> AAAAAAAAAAAAAAAAAAAAAAAAAAAAAAAASLCLFPEDFLLKEFVEFF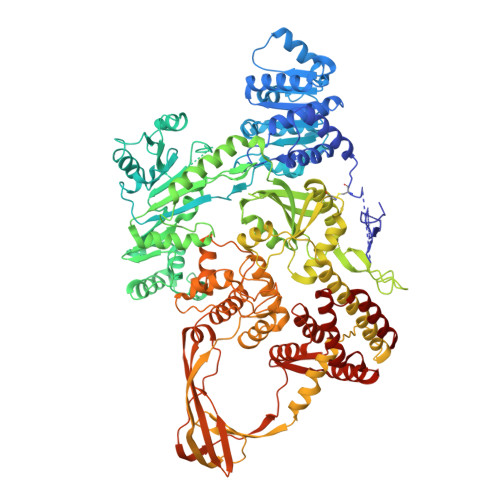RKCVGEPRAIQKMWAKRILRKESFAATAPTGVGKTSFGLAMSLFLALKGKRCYVIFPTSLLVIQAAETIRKYAEKAGVGTENLIGYYHGRIPKREKENFMQNLRNFKIVITTTQFLSKHYRELGHFDFIFVDDVDAILKASKNVDKLLHLLGFHYDLKTKSWVGEARGCLMVSTATAKKGKKAELFRQLLNFDIGSSRITVRNVEDVAVNDESISTLSSILEKLGTGGIIYARTGEEAEEIYESLKNKFRIGIVTATKKGDYEKFVEGEIDHLIGTAHYYGTLVRGLDLPERIRFAVFVGCPSFRVTIEDIDSLSPQMVKLLAYLYRNVDEIERLLPAVERHIDEVREILKKVMGKERPQAKDVVVREGEVIFPDLRTYIQGSGRTSRLFAGGLTKGASFLLEDDSELLSAFIERAKLYDIEFKSIDEVDFEKLSRELDESRDRYRRRQEFDLIKPALFIVESPTKARQISRFFGKPSVKVLDGAVVYEIPMQKYVLMVTASIGHVVDLITNRGFHGVLVNGRFVPVYASIKRCRDCGYQFTEDRESCPKCGSENVDNSRSRIEALRKLAHDAEFVIVGTDPDTEGEKIAWDLKNLLSGCGAVKRAEFHEVTRRAILEALESLRDVDENLVKAQVVRRIEDRWIGFVLSQKLWERFNNRNLSAGRAQTLVLGWIIDRFQESRERRKIAIVRDFDLVLEHDEEEFDLTIKLVEEREELRTPLPPYTTETMLSDANRILKFSVKQTMQIAQELFENGLITYHRTDSTRVSDVGQRIAKEYLGDDFVGREWGESGAHECIRPTRPLTRDDVQRLIQEGVLVVEGLRWEHFALYDLIFRRFMASQCRPFKVVVKKYSIEFDGKTAEEERIVRAEGRAYELYRAVWVKNELPTGTFRVKAEVKSVPKVLPFTQSEIIQMMKERGIGRPSTYATIVDRLFMRNYVVEKYGRMIPTKLGIDVFRFLVRRYAKFVSEDRTRDLESRMDAIERGELDYLKALEDMYAEIKSID>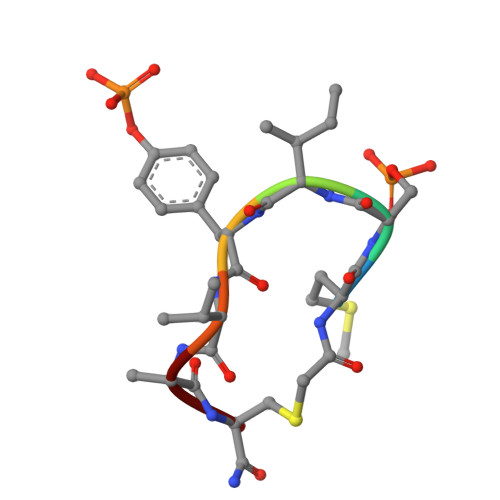 MSIYVAX>MHHHHHHSAEQIMRDRSELARKGIARGRSVVVLTFRDGVLFVAENPSTALHKVSELYDRLGFAAVGKYNEFENLRRAGIVHADMRGYSYDRRDVTGRSLANAYAQTLGTIFTEQPKPYEVEICVAEVGRVGSPKAPQLYRITYDGSIVDEQHFVVMGGTTEPIATAMRESYRADLDLEAAVGIAVNALRQGGAGEGEKRNVDVASLEVAVLDQSRPRRAFRRIAGTALEQLVPAEPAAASESAPEPKPDTETKPADTQD[7x];>[7x]MTADRPALRTGDRDTRLSFGSNLSSFTDYLRGHAPELLPENRIGHRSHSTRGGDGMESGDLAPHGTTIVALTYKGGVLLAGDRRATQGNLIASRDVEAVYVTDEYSAAGIAGTAGIAIELVRLFAVELEHYEKIEGVPLTFDGKANRLASMVRGNLGAAMQGLAVVPLLVGYDLDADDESRAGRIVSYDVVGGRYEERAGYHAVGSGSLFAKSALKKIYSPDSDEETALRAAIESLYDAADDDSATGGPDLTRGIYPTAVTITQAGAVHVSEETTSELARRIVAERTEQ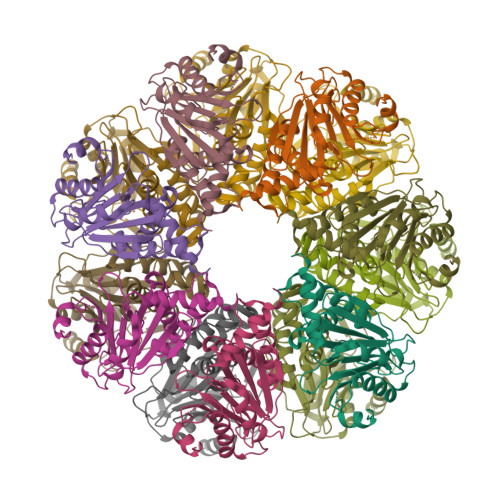GGSAR>SNAYKMESRIKDISLAEFGLQDMEIAKTDMMGLVELQRKYRDSKPLKGARITGSLHLTIETSVLVETLYELGAEIRWCSCNIYSTQDHAAAALVKKNIATVFAWKNETIEDYWVCLNDAMTWRNPNDKDKICGPNLIVDDGGDATLILHEGVKAEIEYEKYNKIPEYLETELDENGKQLSMDLKCMYKVLKMELLKNPFRWRGMLKDLYGVSEETTTGVLRLKIMESEGKLLLPAINVNDSVTKSKFDNTYGCRQSLLHGLFNGCIQMLAGKKIVVLGYGEVGKGCAQGLSGVGARVIVTEIDPICALQASMEGYQVSVLEDVVSEADIFITATGNKDVITVEHMRKMKENAYIANIGHFDDEIDVYGLENYPGIKVIEVKQNVHKFTFPDTQKSVILLCKGRLVNLGCATGHPPLVMSMSFTNQVLAQMDLWKSRELVDRSKNTRFFV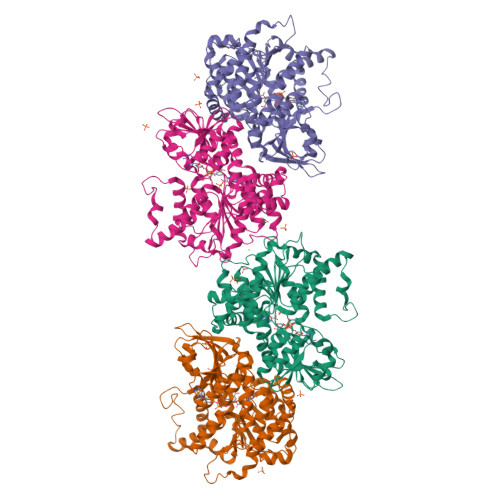KKLSKELDEYVARLHLDVLGIKLTKLTETQAKYINVSINGPYKSEDYRY[4x]> GSHMVPAALPQLTPTLVSLLEVIEPEVLYAGYDSSVPDSAWRIMTTLNMLGGRQVIAAVKWAKAIPGFRNLHLDDQMTLLQYSWMSLMVFALGWRSYRQASGNLLCFAPDLIINEQRMTLPCMYDQCKHMLFISTELQRLQVSYEEYLCMKTLLLLSSVPKEGLKSQELFDEIRMTYIKELG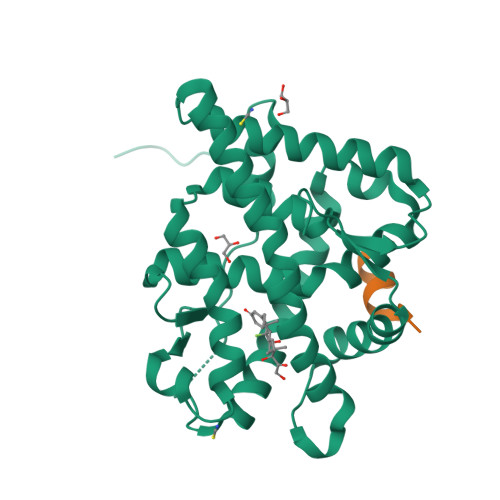KAIVKREGNSSQNWQRFYQLTKLLDSMHDVVENLLSYCFQTFLDKSMSIEFPEMLAEIITNQIPKYSNGNIKKLLFHQK;> KENALLRYLLDKD>[4x]GEIYTETLQQTYAWTAGTNIPIKIPRNNFIRKIRVQLIGSISNSGTAAVTLPSAPFPYNLVQTFNLSYEGSKTLYSVSGTGLGILMYYTTKGQNPAYPAPGTSVPASGSVNLNVMWEFDLARFPATMVQNIILSILTGQAPSGVSINASFYITITYERVTAQEILSEGGLGADGEMPLATVLPKVIEIPTFNV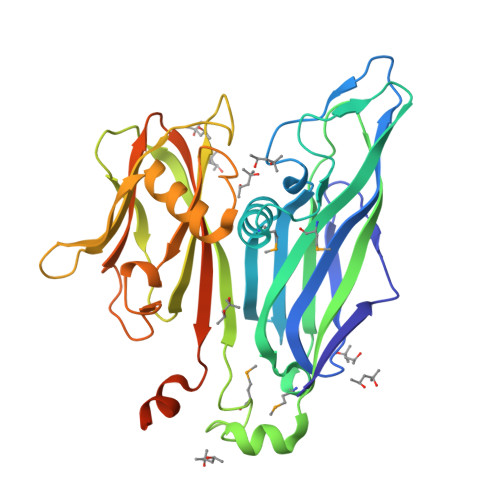PASSAPIHVAYLQPGQIYKRQLVYVINSTSGINNTDPTEYELKIVRGVPTDKIKVSWAALQAENQAEYQVAPYSGASAIIDFRKYFNGDLDLTHAPSDSIEYDLALQNQDNVYSLYVSYVLPYYDQLAALPAQVAAIVQQYVARQKRRIKRHHHHHH> MRVKVIDADAFSYIFRTLEEFIDEITLDFTSDGLKI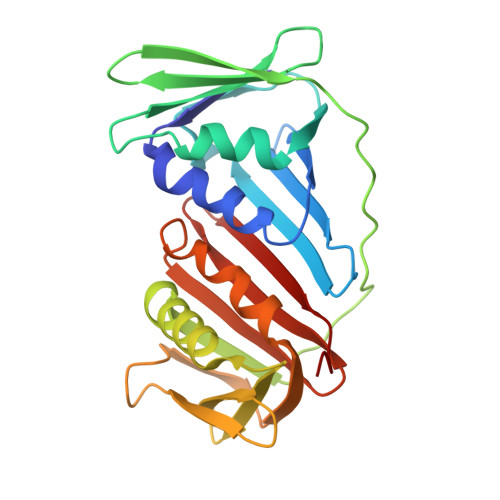RGIDPSRVTFIDILIPAGYFEEYNVEKEEKVGVKLEDFTDVLKTVTKNDSLYLETDENQNIKVTLDGVYERTFTFPSIVASEIETPNLNLEFPFKAKALTVTFTDIIDEIEDIGGDSITFKAEGGKLYLSANSDMGSSTIELSTENGGLLESEGGDAESVYGLEYVVNTSKMRKPSDTVEIAFGSQIPLKLRYNLPQGGYADFYIAPRAE>[2x]MGVDPFQVAVGVSNRHIHLSRTDMDTLFGPGAELQRKKAMKQPGQFAAEETVTLKGPKGSLSKVRVLGPLRRETQVEVSVADGFALGITPPLRQSGQLDDTPGLTIIGPQGSVTKDHGVIVAQRHIHMHPSTAAKLGLRNGDEVDVEAGGERGGVMHRVLIRVAEASADEMHIDVEEANALCLKNDDVVRICKKLEHHHHHH

More recently, a second type of PTAC without any sequence homology to Pta was identified. This protein, PduL (Pfam domain PF06130), was shown to catalyze the conversion of propionyl-CoA to propionyl-phosphate and is associated with a BMC involved in propanediol utilization, the PDU BMC. Not only does PduL facilitate substrate level phosphorylation, but it also is critical for cofactor recycling within, and product efflux from, the organelle. Structurally, PduL consists of two domains (blue/red), each a beta-barrel that is capped on both ends by short α-helices. β-Barrel 1 consists of the N-terminal β strand and β strands from the C-terminal half of the polypeptide chain (β1, β10-β14; residues 37–46 and 155–224). β-Barrel 2 consists mainly of the central segment of primary structure (β2, β5–β9; residues 47–60 and 82–154) (red), but is interrupted by a short two-strand beta sheet (β3-β4, residues 61–81). The active site of PduL is formed at the interface of the two structural domains.

We collected a native dataset from rPduLΔEP crystals diffracting to a resolution of 1.54 Å. A CoA cofactor as well as two metal ions are clearly resolved in the density (for omit maps of CoA see S2 Fig). CoA and the metal ions bind between the two domains, presumably in the active site. The first zinc ion (Zn1) is in a tetrahedral coordination state with His48, His50, Glu109, and the CoA sulfur. The second (Zn2) is in octahedral coordination by three conserved histidine residues (His157, His159 and His204) as well as three water molecules. The interface between the two chains buries 882 Å2 per monomer and is mainly formed by α-helices 2 and 4 and parts of β-sheets 12 and 14, as well as a π–π stacking of the adenine moiety of CoA with Phe116 of the adjacent chain. Our PduL crystals contained CoA that was captured from the Escherichia coli cytosol, indicating that the “ground state” of PduL is in the CoA-bound form; this could provide an elegantly simple means of guaranteeing a 1:1 ratio of CoA:PduL within the metabolosome lumen. The free CoA-bound form is presumably poised for attack upon an acyl-phosphate, indicating that the enzyme initially binds CoA as opposed to acyl-phosphate. This hypothesis is strengthened by the fact that the CoA-bound crystals were obtained without added CoA, indicating that the protein bound CoA from the E. coli expression strain and retained it throughout purification and crystallization. SEC-MALS analysis of rPdulΔEP is consistent with a dimer (as observed in the crystal structure) with a weighted average (Mw) and number average (Mn) of the molar mass of 58.4 kDa +/− 11.2% and 58.8 kDa +/− 10.9%, respectively. rPduL full length runs as Mw = 140.3 kDa +/− 1.2% and Mn = 140.5 kDa +/− 1.2%.> MTTACPARTSSLMDDLLGLLRIRIKRGVNLAVRDISSSDPYVVVKMGKQKLKTRVINKDVNPEWNEDLTLSVTDSNLTVLLTVYDHDMFSKDDKMGDAEFEISPYIEALRMQLDGLPSGTIVTTVKPSRRNCLAEESRVTWVDGKLVQDLVL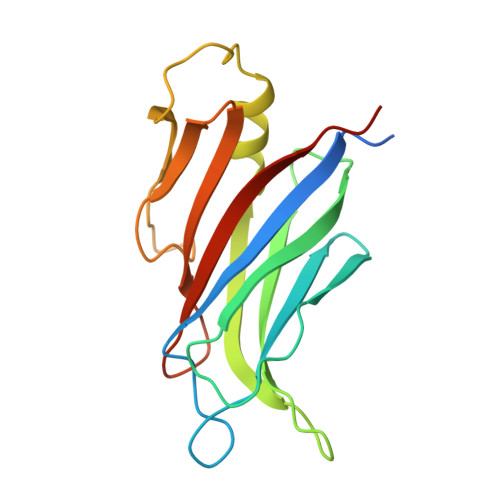RLRHVECGEVEAQLQWIDLPGSKGL>[2x]GAMGMLQQIRGPADLQHLSQAQLRELAAEIREFLIHKVAATGGHLGPNLGVVELTLALHRVFDSPHDPIIFDTGHQAYVHKMLTGRSQDFATLRKKGGLSGYPSRAESEHDWVESSHASAALSYADGLAKAFELTGHRNRHVVAVVGDGALTGGMCWEALNNIAASRRPVIIVVNDNGRSYAPTIGGVADHLAG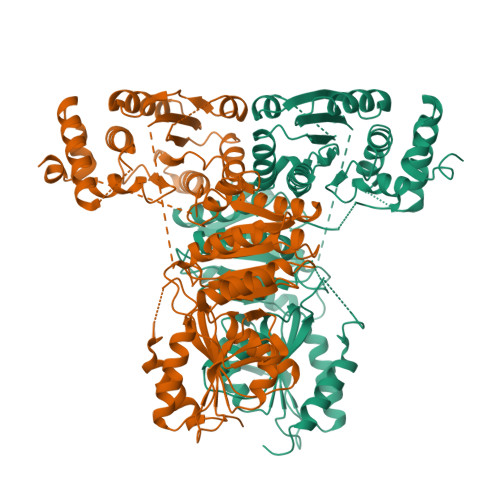GGGGGGPQLLFTDLGLKYVGPVDGHDERAVEVALRSARRFGAPVIVHVVTRKGMGYPPAEADQAEQMHSTVPIDPATGQATKVAGVGWTATFSDALIGYAQKRRDIVAITAAMPGPTGLTAFGQRFPDRLFDVGIAEQHAMTSAAGLAMGGLHPVVAIYSTFLNRAFDQIMMDVALHKLPVTMVLDRAGITGSDGASHNGMWDLSMLGIVPGIRVAAPRDATRLREELGEALDVDDGPTALRFPKGDVGEDISALERRGGVDVLAAPADGLNHDVLLVAIGAFAPMALAVAKRLHNQGIGVTVIDPRWVLPVSDGVRELAVQHKLLVTLEDNGVNGGAGSAVSAALRRAEIDVPCRDVGLPQEFVEHASRSEVLADLGLTDQDVARRITGWVAALGTGVCASDAIPEHLD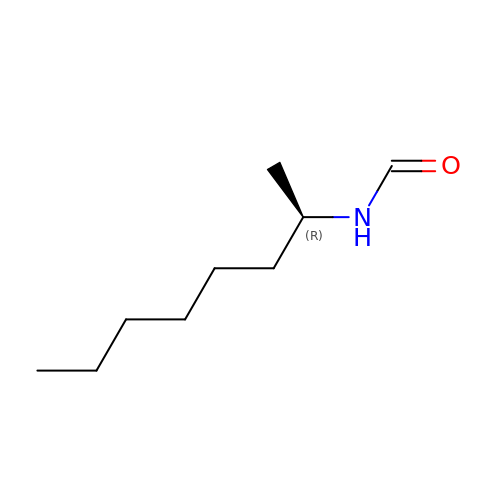1-METHYLHEPTYLFORMAMIDE | C9 H19 N O | YWFHDUFNGSJLTL-SECBINFHSA-N D-sorbose 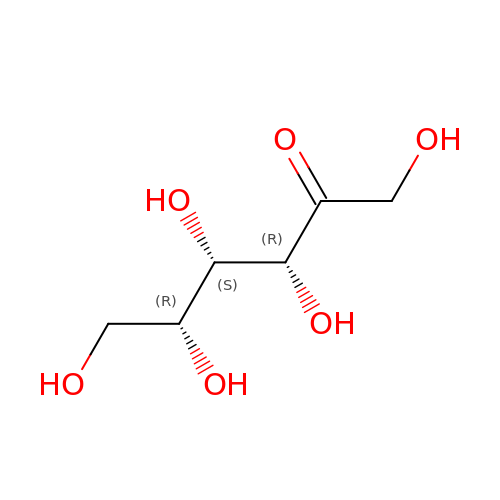| C6 H12 O6 | BJHIKXHVCXFQLS-PYWDMBMJSA-N>MAKLLIMSIVSFCFIFLLLLFFRYILKRYFNYMLNYKVWYLTLLAGLIPFIPIKFSLFKFNNVNNQAPTVESKSHDLNHNINTTKPIQEFATDIHKFNWDSIDNICTVIWIVLVIILSFKFLKALLYLKYLKKQSLYLNENEKNKIDTILFNHQYKKNIVIRKAETIQSPITFWYGKYIILIPSSYFKSVIDKRLKYIILHEYAHAKNRDTLHLIIFNIFSIIMSYNPLVHIVKRKIIHDNEVEADRFVLNNINKNEFKTYAESIMDSVLNVPFFNKNILSHSANGKKSLLKRRLINIKEANLKKQSKLILIFICIFTFLLMVIQSQFLMGQSITDYNYKKPLHNDYQILDKSKIFGSNSGSFVMYSMKKDKYYIYNEKESRKRYSPNSTYKIYLAMFGLDRHIINDENSRMSWNHKHYPFDAWNKEQDLNTAMQNSVNWYFERISDQIPKNYTATQLKQLNYGNKNLGSYKSYWMEDSLKISNLEQV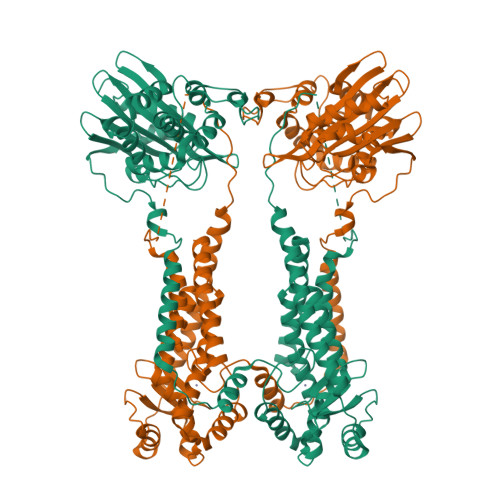IVFKNMMEQNNHFSKKAKNQLSSSLLIKKNEKYELYGKTGTGIVNGKYNNGWFVGYVITNHDKYYFATHLSDGKPSGKNAELISEKILKEMGVLNGQELALVPRGSSAHHHHHH[2x]>[4x]MKRKLIVAVVCLIFICFGINTPAHATSVVSIPINNAGFEDPFIEVVDDYTVDTPPGWTTYNPNNL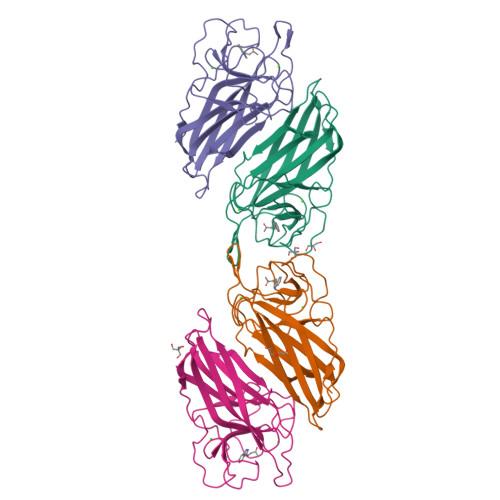VPEKRTTWTSNNGVGYVGPGTQFYNQLAPEGRNIGYIYLAQKPGSGVAGFEQILDATLEPDTNYTLKVDVGNLAGTFKGLSFAGFPGYRVELLAGDTVLAADHNNLFIKEGEFKTSTVTYTSTAKDLHLGQKLGIRLVNLLQDKFSGLDFDNVRLTAEPTEA> MLSPKAATLAERSAGLAFSLYQAMAKDQAVENILLSPVVVASSLGLVSLGGKATTASQAKAVLSAEQLRDEEVHAGLGELLRSLSNSTARNVTWKLGSRLYGPSSVSFAEDFVRSSKQHYNCEHSKINFRDKRSALQSINEWAAQTTDGKLPEVTKDVERTDGALLVNAMFFKPHWDEKFHHKMVDNRGFMVTRSYTVGVTMMHRTGLYNYYDDEKEKLQIV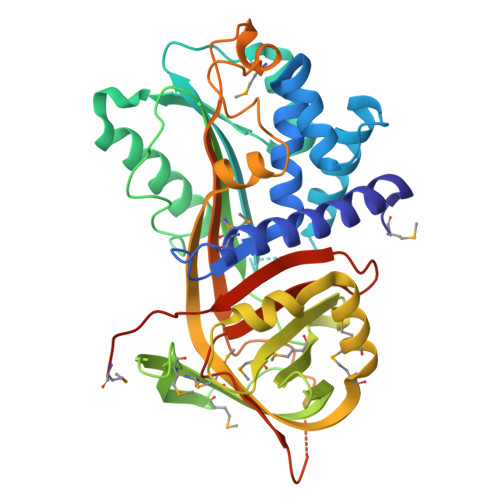EMPLAHKLSSLIILMPHHVEPLERLEKLLTKEQLKIWMGKMQKKAVAISLPKGVVEVTHDLQKHLAGLGLTEAIDKNKADLSRMSGKKDLYLASVFHATAFEWDTEGNPFDQDIYGREELRSPKLFYADHPFIFLVRDTQSGSLLFIGRLVRPKGDKMRDELLEHHHHHH>[2x]MAHHHHHHMSEYLFTSESVS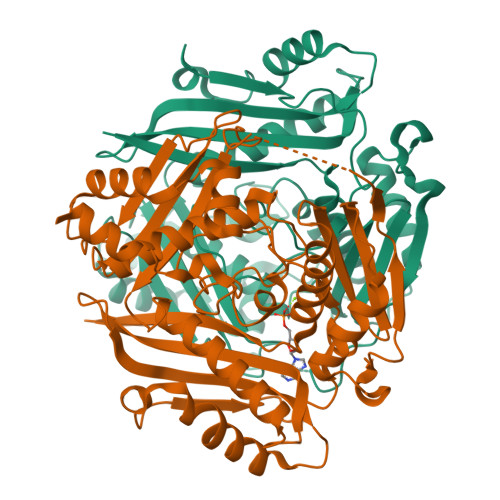EGHPDKVADQVSDAILDAILAQDPKARVAAETLVNTGLCVLAGEITTTAQVDYIKVARETIKRIGYNSSELGFDANGCAVGVYYDQQSPDIAQGVNEGEGIDLNQGAGDQGLMFGYACDETPTLMPFAIYYSHRLMQRQSELRKDGRLPWLRPDAKAQLTVVYDSETGKVKRIDTVVLSTQHDPAISQEELSKAVIEQIIKPVLPPELLTDETKYLINPTGRFVIGGPQGDCGLTGRKIIVDTYGGAAPHGGGAFSGKDPSKVDRSAAYACRYVAKNIVAAGLATQCQIQVSYAIGVAEPTSISIDTFGTGKISEEKLIALVCEHFDLRPKGIVQMLDLLRPIYGKSAAYGHFGREEPEFTWERTDKAASLKAAAGL> DMPVERILEAELAVEPKTETYVEANMGLNPSSPNDPVTNICQAADKQLFTLVEWAKRIPHFSELPLDDQVILLRAGWNELLIASFSHRSIAVKDGILLATGLHVHRNSAHSAGVGAIFDRVLTELVSKMRDMQMDKTELGCLRAIVLFNPDSKGLSNPAEVEALREKVYASLEAYCKHKYPEQPGRF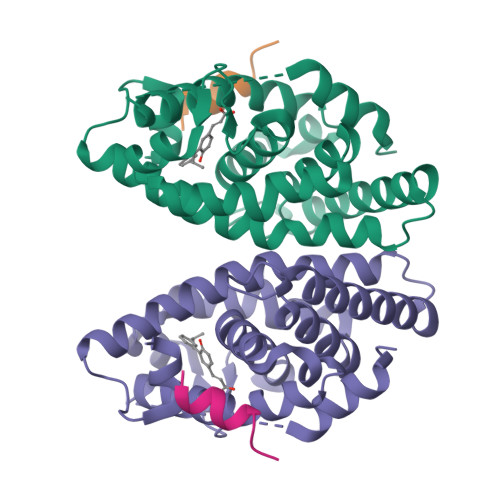AKLLLRLPALRSIGLKCLEHLFFFKLIGDTPIDTFLMEMLE;> HKILHRLLQDS> MSIPNSFIIVGSGVFGLSLAYALSLDDRFADKKIILVDRWNFEPPNATGSVHNPAAANADTSRVIRRDYPHGPYASLALEAMKHWRGKFGENNRYVNQRLLFSGEGSSLTTPPKALETVNYIKKAYAISCELTPGGRDAVQVLDSLDEVRAFLGNTPSHPPHLPVNKDPAARDLRGYVSNDCGWADAGASIEWLRQEVLRLGRVECVVGEVESLVYSDDQRAVKGVKLVDGKVLTAELTVIAAGARSSHILGIPKLCDVYSEFVAYIQLTKEEADELRRRQWPILVNCHRGVFAVGPDHDNCLKFGHFSYSGIVDVLREASIQVPTRPDGWEAQQKYWSDPRFAFGGEVKVSALGDVDDYENPAAQRALADYRLFLL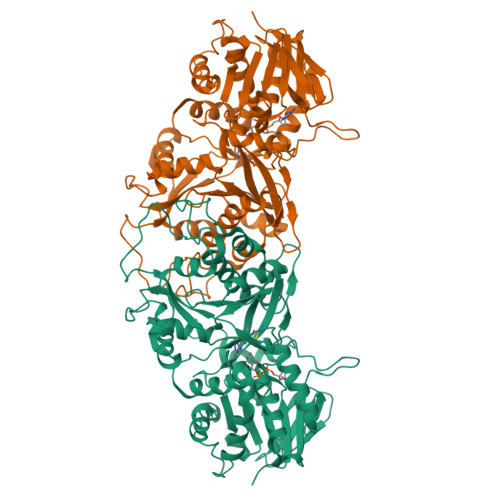ELLGPTGLQGVDTLGLDQSDNLLNNIANRPFTRVRKCWYNDTPALDFVVDYHPSYGKTLFVATGGCDHAFKFLPIIGEKTLALILRNRGDSAVSLPAGVEPSLEELSELWRFPVELLQDN Asparaginases (EC 3.5.1.1), which split L-asparagine to L-aspartate and ammonia, are grouped into three unrelated structural classes: Class 1 (bacterial-type), Class 2 (plant-type), and Class 3 (Rhizobium etli-type). ReAV is a homodimer with an α/β protomeric fold, formed by two tightly packed domains. The active site of the enzyme is located in a cleft on the protomer surface and marked by a zinc ion with an unusual coordination sphere created by Cys135, Lys138, Cys189, and a water molecule. The conspicuous catalytic center of the enzyme comprises two Ser-Lys tandems (Ser48-Lys51 and Ser80-Lys263), centered around the curiously hydrated Ser48 residue and located in the close vicinity of the metal binding site.

The ReAV D187A crystal structure revealed that the absence of Asp187 induced only small local conformational changes and atomic shifts, and these changes are strictly equivalent in the two dimers. The zinc cation is only partially present at the metal binding site, with a refined occupancy of 0.5, as is the w1 water molecule from the metal coordination sphere. Moreover, substitution of Asp187 with alanine affected the metal environment, since a sulfate ion occurs right next to the strongly bound water molecule from the zinc coordination sphere. The sulfate ion fills a central position in the active site cleft, possibly preventing the enzyme from accepting a substrate molecule. The negatively charged SO4 2- anion forms a salt bridge with the protonated and positively charged side chain of Arg47. The hydration pattern of Ser48 is nearly identical as in the WT protein, with three closely-spaced water molecules in the vicinity of the Ser48 hydroxyl group. Surprisingly, the side chain of Cys249 is not oxidized to sulfenic acid, which may be related to a change in the zinc environment. Although Ser48 remained hydrated in the D187A mutant, the mutation completely abolished the enzymatic activity, despite the fact that this mutein can still bind zinc (KD of 7.2 μM). This observation may be correlated with the presence of the sulfate ion in the active site, which would hinder the acceptance of a genuine substrate molecule. We hypothesize that with altered metal binding properties, the coordination site of the D187A mutant could become specific for other transition metal ions, which could be bound during protein bacterial expression or purification on Ni2+ resin.

>[4x]GIDPFTMTPSEDFVVTDRGGIVENSHRVHAAVVDAKGRLLYALGNPTRMTLARSAAKPAQALAILETEGVAGYGFDDADIALMCASHSSEDRHIARTRAMLSKIKAEEADLRCGGHPSLSEMVNRSWIKQDFIPTAVCSNCSGKHVGMLAGARAIGAGTDGYHLPDHPMQGRVKRTVAELCDLDAGDVEWGTAGCNLPTPAFPLDRLGRIYAKLASAADGSDAGEGQSTRCAALAHIFRAMARHPEMVAGEGRYCTMLMRAFDGALVGKLGADASYAIGVRASDATRQLGTDGALGISVKIEDGNLEMLYAVVTELLERLGIGSPDVRSQLASFHHPQRVNTMGVTTGGVSFPFKLRGSKSNVDDPRLAAVAR(2S)-4-(5-chloro-1,3-benzoxazol-2-yl)-1-(N,3-dicyclohexyl-D-alanyl)-N-[(thiophen-2-yl)methyl]piperazine-2-carboxamide | C32 H42 Cl N5 O3 S | 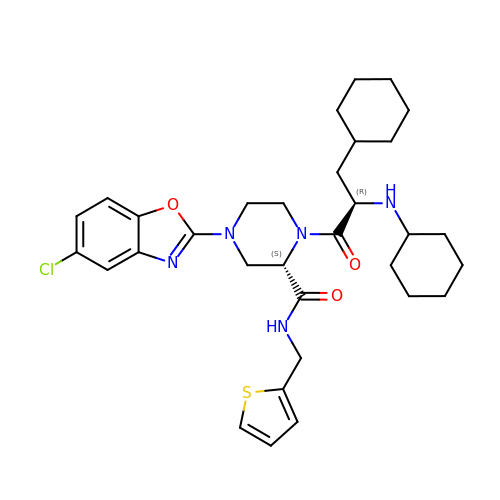WQMFHHFJPDQBMH-IZLXSDGUSA-N> APDSVDYRKKGYVTPVKNQGQCGSCWAFSSVGALEGQLKKKTGKLLNLAPQNLVDCVSENDGCGGGYMTNAFQYVQKNRGIDSEDAYPYVGQEESCMYNPTGKAAKCRGYREIPEGNEKALKRAVARVGPVSVAIDASLTSFQFYSKGVYYDESCNSDNL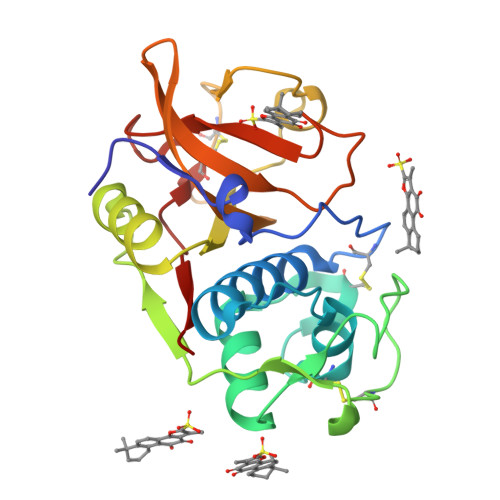NHAVLAVGYGIQKGNKHWIIKNSWGENWGNKGYILMARNKNNACGIANLASFPKM2-(5-AMINO-6-OXO-2-M-TOLYL-6H-PYRIMIDIN-1-YL)-N-[4-GUANIDINO-1-(THIAZOLE-2-CARBONYL)-BUTYL]-ACETAMIDE | C22 H26 N8 O3 S | 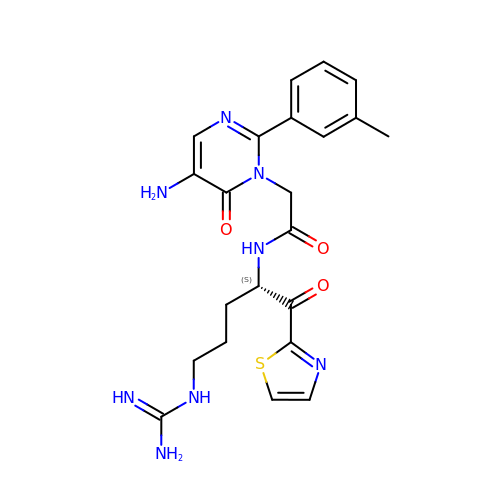WNJLVFWJWNGWKN-INIZCTEOSA-N PHOSPHORIC ACID MONO-[5-(2-AMINO-4-OXO-4,5-DIHYDRO-3H-PYRROLO[3,2-D]PYRIMIDIN-7-YL)-3,4-DIHYDROXY-PYRROLIDIN-2-YLMETHYL] 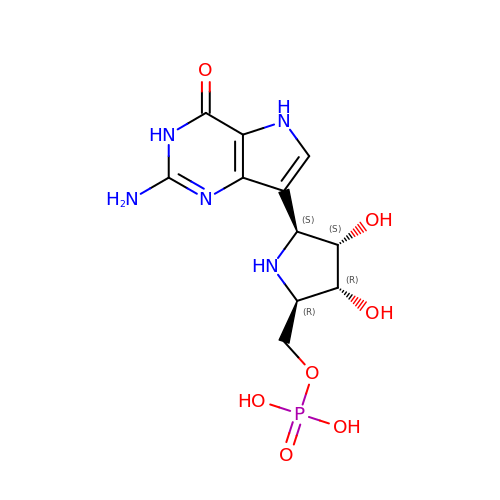ESTER | C11 H16 N5 O7 P | IQLBECLICFDTTF-PVEDRDFWSA-N>[2x]MASSMRSLFSDHGKYVESFRRFLNHSTEHQCMQEFMDKKLPGIIGRIGDT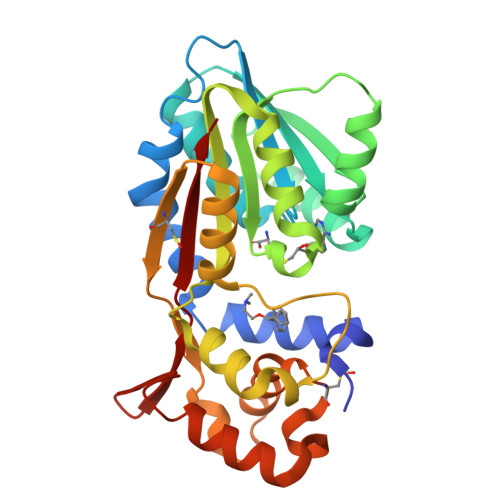KSEIKILSIGGGAGEIDLQILSKVQAQYPGVCINNEVVEPSAEQIAKYKELVAKTSNLENVKFAWHKETSSEYQSRMLEKKELQKWDFIHMIQMLYYVKDIPATLKFFHSLLGTNAKMLIIVVSGSSGWDKLWKKYGSRFPQDDLCQYITSDDLTQMLDNLGLKYECYDLLSTMDISDCFIDGNENGDLLWDFLTETCNFNATAPPDLRAELGKDLQEPEFSAKKEGKVLFNNTLSFIVIEA> GMIDLDFRKLTIEECLK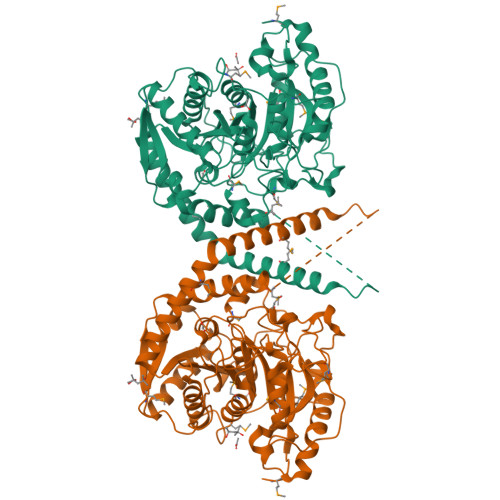LSEEEREKLPQLSLETIKRLDPHVKAFISVRENVSVEKKGKFWGIPVAIKDNILTLGMRTTCASRILENYESVFDATVVKKMKEAGFVVVGKANLDEFAMGSSTERSAFFPTRNPWDLERVPGGSSGGSAAAVSAGMVVAALGSDTGGSVRQPASLCGVVGYKPTYGLVSRYGLVAFASSLDQIGPITKTVRDAAILMEIISGRDENDATTVNRKVDFLSEIEEGVSGMKFAVPEEIYEHDIEEGVSERFEEALKLLERLGAKVERVKIPHIKYSVATYYVIAPAEASSNLARFDGVKYGLRIKEKGLREMYMKTRNVGFGEEVRRRIMIGTFTLSAAYYEAYFNKAMKVRRKISDELNEVLSQYDAILTPTSPVTAFKIGEIKDPLTYYLMDIFTIPANLAGLPAISVPFGFSNNLPVGVQVIGRRFADGKVFRIARAIEKNSPYNENGMFPLPEVKA We show that the orthologue identified in A. hydrophila (AhlABC) is a haemolytic tripartite α-PFT, requiring all three components for maximal lysis, and we present the structures of the soluble forms of monomeric AhlB and tetrameric AhlC and the decameric pore form of AhlB. AhlC provides the initial single leaflet insertion, assembly with AhlB then producing an oligomeric hydrophobic pore, and finally recruitment of AhlA produces a hydrophilic fully active AhlABC pore. Structural and sequence analysis suggests this method of pore assembly may well occur throughout the tripartite α-PFT family.

We have also determined the structure of a second crystal form of soluble AhlC in space group P21, which contains a complete tetramer in the asymmetric unit. In this second crystal form the head domains of subunit Q and S do not form crystal contacts and the electron density for these areas is poor, indicating that these hydrophobic head domains are flexible within the tetramer. Flexibility of the head to disassociate from the tetramer when presented with a hydrophobic surface is also shown in the crystals of AhlC, where the α3–α4 hydrophobic heads of two subunits protrude from the tetramer to pack against equivalent regions of symmetry related molecules in one crystal form and make no contacts and are disordered in the other. However, the AhC subunits of the soluble tetramer adopt a pore type conformation with the hydrophobic heads buried within the tail domains of symmetry related subunits. Thus some disassembly of the AhlC tetramer must occur before membrane attachment, supported by the cross-linking of AhlC, which abolishes lytic activity. To determine if disassembly of the tetramer is required for membrane binding, we cross-linked soluble AhlC with glutaraldehyde to produce equal proportions of AhlC monomer and AhlC dimer, whereas when AhlC was cross-linked with both glutaraldehyde and 1-ethyl-3-(3-dimethylaminopropyl)carbodiimide, the dimeric species was formed exclusively. Haemolytic assays using these cross-linked samples showed that lysis was abolished for the purely dimeric form and reduced by about 50% for the mixture of monomeric and dimeric AhlC.

>[4x]MSNGILSQSIANMQQAEATIQSFSGLPQNAVNIQQNVGEVVAALLPQVQTMQQQVLAFAARLELQLTQQLANTGPFNPEALKAFVDLVQQEIAPIQTLTAQTLTASQSANDRITQDNIALQRIGVELQATIAGLQSNLDGARQELDSLNKKKLYLLGLGLLGLPGLIALAVTLTQTQNKVSSLEGQVNQIEGQIQRQQGFLGQTTAFSQQFGSLIDRVSKVGNTISLLGGDIANVARDAGQGDPELARLFFTAALTEVRTLQVDASLEHHHHHH>GSHMGLQGPSGAADKAGTRENQP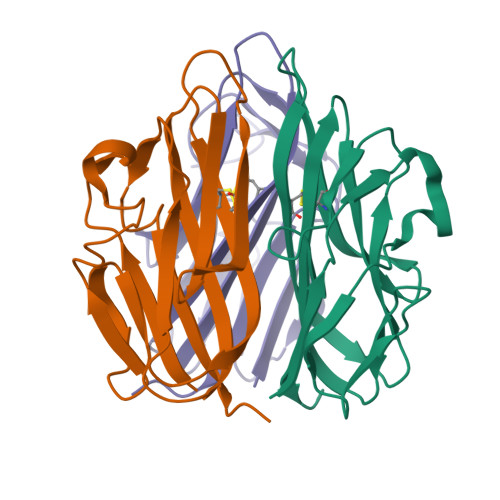AVVHLQGQGSAIQVKNDLSGGVLNDWSRITMNPKVFKLHPRSGELEVLVDGTYFIYSQVYYINFTDFASYEVVVDEKPFLQCTRSIETGKTNYNTCYTAGVCLLKARQKIAVKMVHADISINMSKHTTFFGAIRLGEAPAS[6x]>[3x]TTILVVRRNGQTVMGGDGQVTFGSTVLKGNARKVRKLGEGKVLAGFAGSVADAMTLFD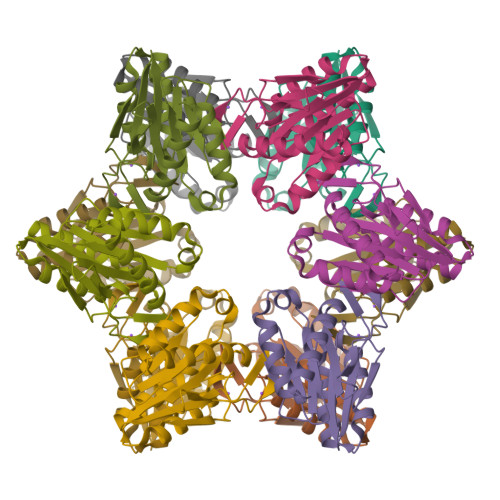RFEAKLREWGGNLTKAAVELAKDWRTDRVLRRLEALLLVADKENIFIISGNGEVIQPDDDAAAIGSGGPYALAAAKALLRNTDLSAREIVEKAMTIAGEICIYTNQNIVIEEV>[6x]GALSVHMDMASVTKAMAAPESGLEVRDRMWLKITIPNAFLGSDVVDWLYHHVEGFPER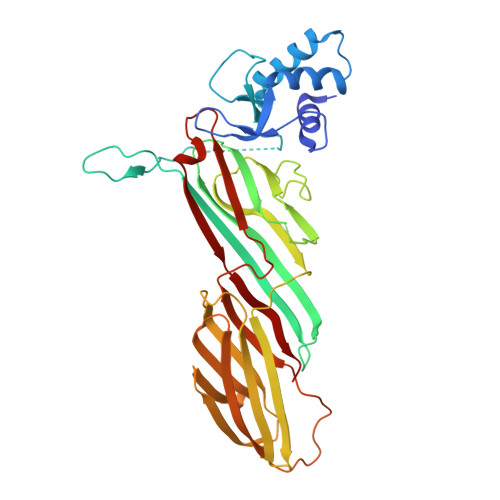REARKYASGLLKAGLIRHTVNKITFSEQCYYVFGDLSGGPRPYSPQPPPYHELEFGGSGGSRNELFLDVLESVNLLMSPQGQVLSAHVSGRVVMKSYLSGMPECKFGMNDKIVIEKQGKGTADETSKSGKQSIAIDDCTFHQCVRLSKFDSERSISFIPPDGEFELMRYRTTKDIILPFRVIPLVREVGRTKLEVKVVIKSNFKPSLLAQKIEVRIPTPLNTSGVQVICMKGKAKYKASENAIVWKIKRMAGMKESQISAEIELLPTNDKKKWARPPISMNFEVPFAPSGLKVRYLKVFEPKLNYSDHDVIKWVRYIGRSGIYETRC> SESQTLDKVYQMKSKPRGYCLIINNHNFAKAREKVPKLHSIRDRNGTHLDAGALTTTFEELHFEIKPHDDCTVEQIYEILKIYQLMDHSNMDCFICCILS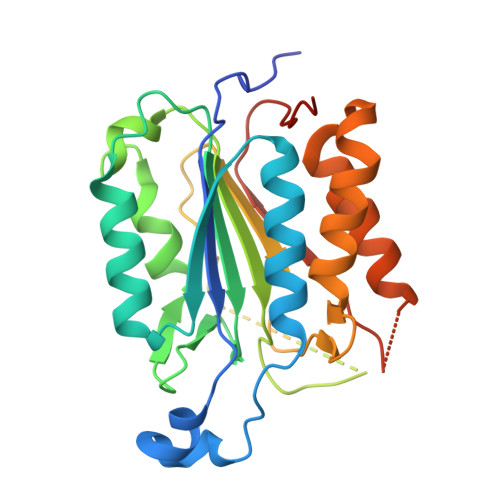HGDKGIIYGTDGQEAPIYELTSQFTGLKCPSLAGKPKVFFIQACQGDNYQKGIPVETASEEQPYLEMALSSPQTRYIPDEADFLLGMATVNNCVSYRNPAEGTWYIQSLCQSLRERCPRGDDILTILTEVNYEVSNKDDKKNMGKQMPQPTFTLRKKLVFPSDVEHHHHHH> TDAKNNLLYFFDRPNEPCFMQKGEDKVVFEIPDHYYPDKYKSLSNTLSNRFGNEATKRIPIRNITLPNLEVPMQLPYNDQFSLFVPKHRTMAAKLIDIFMGMRDVEDLQSVCSYCQLRINPYMFNYCLSVAILHRPDTKGLSIPTFAETFPDKFMDSKVFLRAREVSNVVISGSRMPVNVPINYTANTTEPEQRVAYFREDIGINLHHWHWHLVYPFDSADRSIVNKDRRGELFYYMHQQIIGRYNVERMCNGLPQVKPFSDFSAPIEEGYFPKLDSQVASRTWPPRFAGSVFRNLDRTVDQVKIDVRKLFTWRDQFLEAIQKMAIKMPNGRELPLDEVTGIDMLGNLMESSIISPNRGYYGDLHNMGHVFAAYTHDPDHRHLEQFGVMGDSATAMRDPFFYRWHRFVDDVFNIYKEKLTPYTNERLDFPGVRVSSVGIEGARPNTLRTLWQQSTVELGRGLDFTPRGSVLARFTHLQHDEFQYVIEVNNTTGGNLMGTVRIFMAPKVDDNGQPMSFNKQRRLMIELDKFSQALRPGTNTIRRRSVDSSVTIPYERTFRNQSERPGDPGTAGAAEFDFCGCGWPHHMLIPKGTAQGYPVVLFVMISNWNNDRIEQDLVGSCNDAASYCG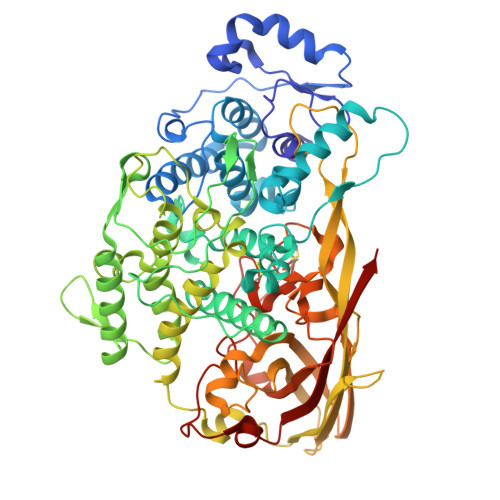IRDRKYPDKQAMGYPFDRKMANDAATLSDFLRPNMAVRDCSIQFSDTTVERGQQG> MEIETIVRESEANRIQAQTWFSHPEKSKVSFRYDERETSSIRSISIETFLSFYSSKFNREPYSVLDIGCGQGQVIQYLNSRFQKIELTGIDSSAQAISSAKKLGINASFICSNAENIMQYVSKKQDIIFIHLCFGLFKNPIAIVNTLIHLLSDQSCIYIVDLDRNSLGEGLNTAQSREEEAYL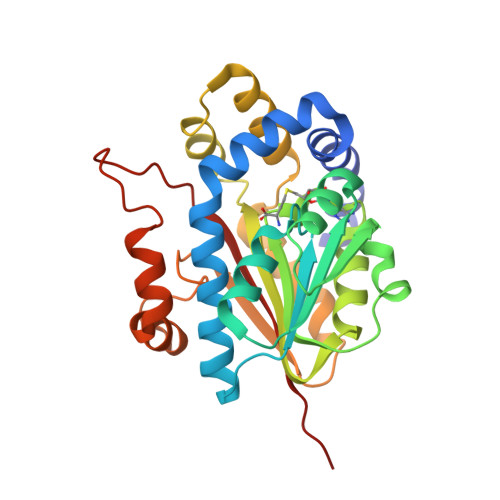KDQYRASLTMEEFKQLLHVVTKEQHGVSFHVGNSFIGGFDETSSQFFSLMRNRNLQDALRTSVGEQLKQSQMPALLHGWIIKNKRYT3-[[1-[(3~{R},4~{R})-1-[5-(3-methoxypyridin-4-yl)thiophen-2-yl]carbonyl-3-phenyl-piperidin-4-yl]carbonyl-4-oxidanyl-piperidin-4-yl]methyl]-7-methyl-pyrrolo[2,3-d]pyrimidin-4-one | C36 H38 N6 O5 S | 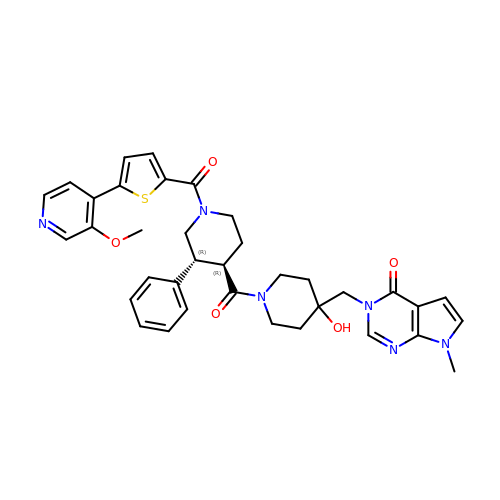YORMIOZUKCOGFP-NAKRPHOHSA-N> NFFQFAEMIVKMTGKEAVHSYAIYGCYCGWGGQGKPQDATDRCCFVHDCCYGTVNDCNPKMATYSYSFENGDIVCGDN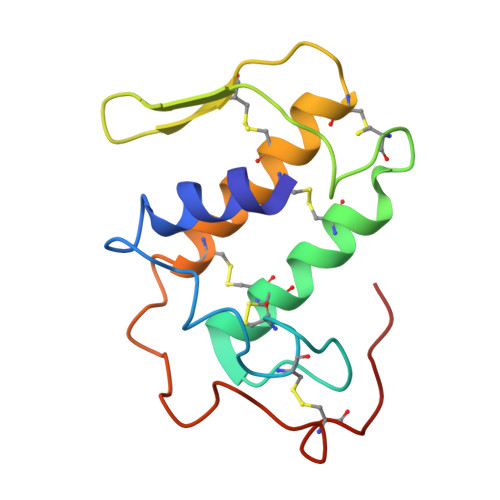NLCLKTVCECDRAAAICLGQNVNTYDKNYENYAISHCTEESEQC>ALVEDNNAVAVSFSEEQEALVLKSWAIL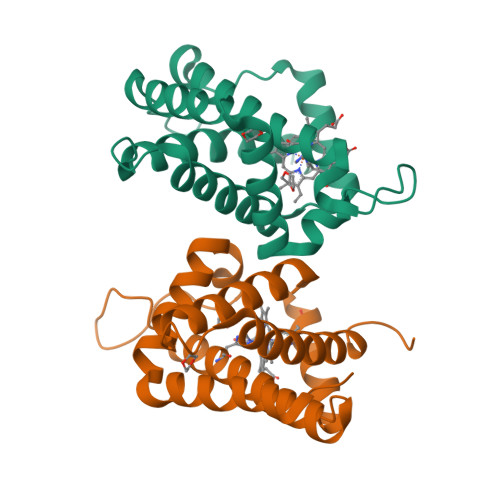KKDSANIALRFLLKIFEVAPSASQMFSFLRNSDVPLEKNPKLKTHAMSVFVMTCEAAAQLRKAGKVTVRDTTLKRLGATHLKYGVGDAHFEVVKFALLDTIKEEVPADMWSPAMKSAWSEAYDHLVAAIKQEMKPAE[2x]> MNPKVLKVGAIPD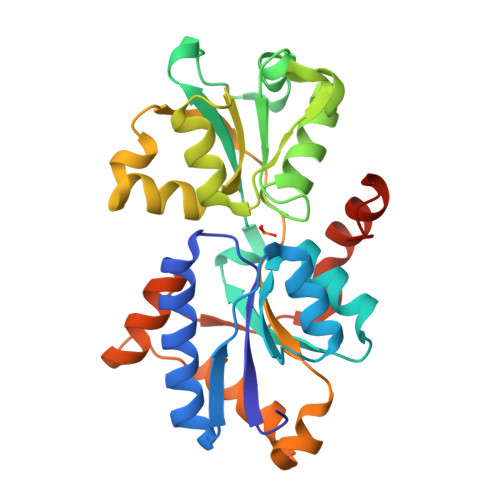QNQDVLDKRFNLFSKELSKQLDVEVKYIPVINYIAAVTGFRTKDLDLVWFGGLSGVQARLQTPNSIVIAQRDIDKEFKSVFVVNKNLELNSISNIKGLKKLKNLRFTFGSENSTSGRLMPEYFLNQAGVEIKHFKGKKAGFSGSHDATIALVNSGAFDAGALNKQVWENNLKNNPKRTSNLELFWITPEYVDYHWVAQGDLENRFGEGFTKELKSVILNLDIKQKSHKQILDMFNAKRFIKAESKQYKNIEEIGRKLNKIRLEHHHHHH>MEGMDPLAVLAESRLLPLLTVRGGEDLLGLARVLEEEGVGALEITLRTEKGLEALKALRKSGLLLGAGTVRSPKEAEAALEAGAAFLVSPGLLEEVAALAQARGVPYLPGVLTPTEVERALALGLSALKFFPAEPFQGVRVLRAYAEVFP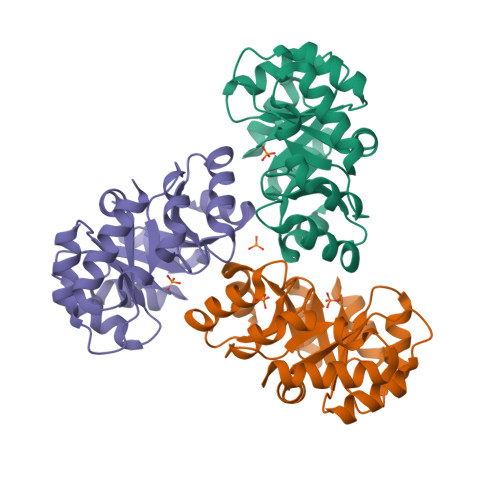EVRFLPTGGIKEEHLPHYAALPNLLAVGGSWLLQGNLEAVRAKVRAAKALLSPQAPG[6x]> PISPIETVPVKLKPGMDGPKVKQWPLTEEKIKALVEICTEMEKEGKISKIGPENPYNTPVFAIKKKDSTKWRKLVDFRELNKRTQDFWEVQLGIPHPAGLKKNKSVTVLDVGDAYFSVPLDEDFRKYTAFTIPSINNETPGIRYQYNVLPQGWKGSPAIFQSSMTKILEPFRKQNPDIVIYQYMDDLYVGSDLEIGQHRTKIEELRQHLLRWGLTTPDKKHQKEPPFLWMGYELHPDKWTVQPIVLPEKDSWTVNDIQKLVGKLNWASQIYPGIKVRQLCKLLRGTKALTEVIPLTEEAELELAENREILKEPVHGVYYDPSKDLIAEIQKQGQGQWTYQIYQEPFKNLKTGKYARMRGAHTNDVKQLTEAVQKITTESIVIWGKTPKFKLPIQKETWE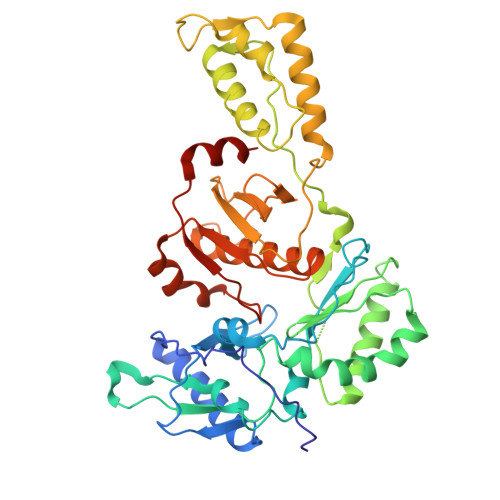TWWTEYWQATWIPEWEFVNTPPLVKLWYQLEKEPIVGAETF> MSSFYTVVGVFIVVSAMSVLFWIMAPKNNQAVWRSTVILTLAMMFLMWAITFLCQLHPLV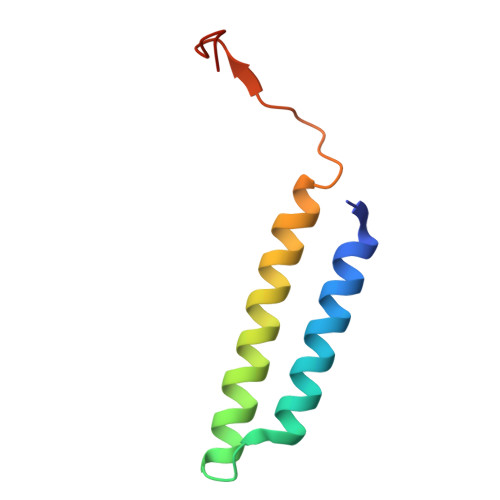APRRSDLRPEFAE>[4x]NSAMEKTLSIIKPDAVKKGVIGKILDRFESNGLRIAAMKKVQLSKEQAENFYAVHKERPFFKDLVEFMISGPVVVSILEGEGAVL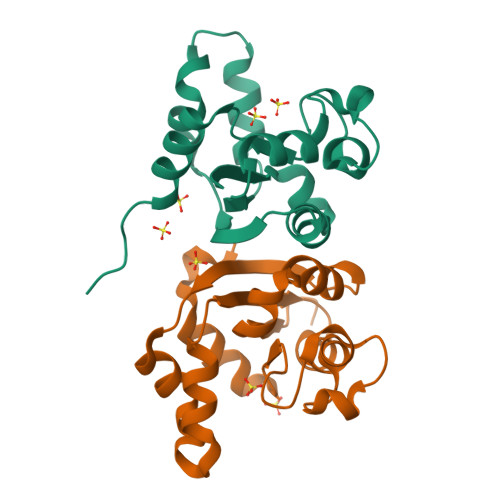KNRDLMGATNPKEAKAGTIRADFAESIDANAVHGSDSLENAKIEIEFFFKPNEIC>MANPVHKITDEKKQQGLEKINSGQRFKANLIKWVSFISGDMAAFGEWMKGQFILLQIMDWVLRGAAQVMFVNNPLSGLIIFAGLILQNRWWALNGFVGTVFATISALILCQNRGAIAAGLYGYNGILVGLLMAVFSNAGDWYWWLLLPNIFMSMACPIVSSALASINSRWDLPVFTLPFNILVCLHMVATGHYNQYFPQILIQPTTSMSNLTWSELDYAQLFRSIPVGIGQVYGCDNAWTGGIFMIALFISSPITFAHATIGSAVGM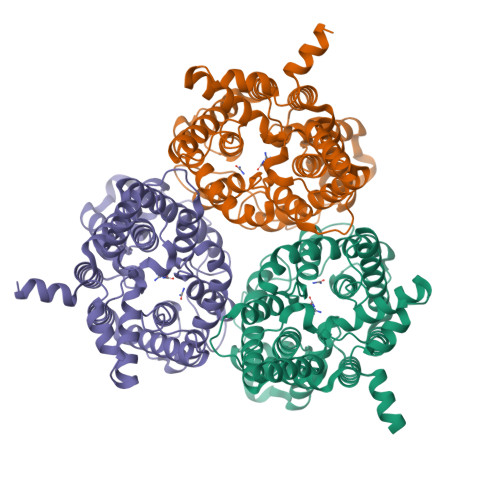VSGLALAAPFKNIYMGLWGYNCVLACIAIGGMFYALTWQTHLLAVACAFFCAYLGSAIGNVMSNFGLPACTWPFCLSALTFLLITTETKFIHKLPLAKVAYPEQNLRYYWKMKKEEKTQKGIQAKDTESQLEKEQISISMEKKDLDICTVDVQQEENTL[3x]> MAETKSMFREVLPKQGQLYVEDITTMVLCKPKLLPLKSLTLEKLEKMQQAAQDTIHQQEMTEKEQKITH;> MAATSSSDSDGGKGESEANSKWLDSLSDSMANIHTFSACLALADFHGDGEYKLAMGDLGPDGRQPRLKVLKGHTLVSQKPLPDLPAAAVTFLMASHEPRTPALAIASGPCVYVYKNLKPYFKFSLPSLPTNPLEQDLWNQAKEDQIDPLTLKEMLEGIREKAEVPLSVQSLRFLPLELSEMEAFVNQHKSKSIRRQTVITTMTTLKKNLADEDAVSCLVLGTENKELLVLDPEAFTILAKMSLPSVPAFLEASGQFDVEFRLAAACRNGSIYILRRDSKRPKYCIELGAQPVGLVGVHKVLVVGSNQDSLHGFTYKGKRLWTVQMPAAILAMNLLEQHSRGLQAVMAALANEEVRIYHDKVLLNVIRTPEAVTSLCFGRYGREDNTLIMTTLGGGLIIKILKRTAVFAEGGGEAGPPPSQAIKLNVPRKTRLYVDQTLREREAGTAMHRTFQADLYLLRLRAARAYVQALESSLSPVSLTAREPLKLHAVVQGLGPTFKLTLHLQNTSTARPILGLVVCFLYNEVLYALPRAFFKVPLLVPGLNYPLETFVKSLSDKGISDIIKVLVLREGQSTPLLSAHINMPMSEGLAAD;> MLQPVFTLKLRHKISPRMVAVGRYDGTHPCLAAATQAGKVFIHNPHSRSQHLGAPRVLQSPLESDVSLLNINQTVSCLTAGVLNPELGYDALLVGTQTNLLAYDVYNNSDLFYREVADGASAIVLGTLGDITSPLAIIGGNCALQGFNHEGNDLFWTVTGDNVHSLALCDFDGDGKKELLVGSEDFDIRVFKEDEIVAEMSETEIITSLCPMYGSRFGYALSNGTVGVYDKTARYWRIKSKNQAMSIHAFDLNSDGVCELITGWSNGKVDARSDRTGEVIFKDNFSSAIAGVVEGDYRMEGCQQLICCSVDGEIRGYLPGTAEMRGNLMDISVEQDLIRELSQKKQNLLLELRNYEENAKAELSSPLNEADGHRGVIPANTKHHTALSVSLGSEAQAAHAELCISTSNDTIIRAVLIFAEGVFAGESHVVHPSVHHLSSSVRIPITPPKDIPVDLHLKTFVGYRSSTQFHVFELTRQLPRFSMYALTSPDPASEPLSYVNFIIAERAQRVVMWLNQNFLLPEDTNIQNAPFQVCFTSLRNGGQLYIKIKLSGEITVNTDDIDLAGDIIQSMASFFAIEDLQVEADFPVYFEELRKVLVKVDEYHSVHQKLSADMADNSNLIRSLLVQAEDARLMRDMKTMKNRYKELYDLNKDLLNGYKIRCNNHTELLGSLKAVNQAIQRAGHLRVGKPKNQVITACRDAIRSNNINMLFRIMRVGTASS;> MAEEKLSARTQLPVSAESQKPVLKKAPEFPILEKQNWLIHLYYIQKDYEACKAVIKEQLQETHGLCEYAIYVQALIFRLEGNIQESLRLFQMCAFLSPQCADNLKQVARSLFLLGKHKAAIEVYNEAAKLNQKDWEICHNLGVCYIYLKQFDKAQDQLHNALHLNRHDLTYIMLGKIFLLKGDLDKAIEIYKKAVEFSPENTELLTTLGLLYLQLGIYQKAFEHLGNTLTYDPTNYKAILAAGSMMQTHGDFDVALTKYKVVACAVIESPPLWNNIGMCFFGKKKYVAAISCLKRANYLAPLDWKILYNLGLVHLTMQQYASAFHFLSAAINFQPKMGELYMLLAVALTNLEDSENAKRAYEEAVRLDKCNPLVNLNYAVLLYNQGEKRDALAQYQEMEKKVNLLKYSSSLEFDPEMVEVAQKLGAALQVGEALVWTKPVKDPKSKHQTASTSKAAGFQQPLGSNQALGQAMSSAATCRKLSSGAGGTSQLTKPPSLPLEPEPTVEAQPTEASAQTREK;> MSVLDALWEDRDVRFDVSSQQMKTRPGEVLIDCLDSVEDTKGNNGDRGRLLVTNLRIVWHSLALPRVNLSIGYNCILNITTRTANSKLRGQTEALYVLTKCNSTRFEFIFTNLVPGSPRLYTSLIAVHRAYETSKMYRDFKLRSALIQNKQLRLLPQENVYNKINGVWNLSSDQGNLGTFFITNVRIVWHANMNDSFNVSIPYLQIRSVKIRDSKFGLALVIESSQQSGGYVLGFKIDPVEKLQESVKEINSLHKVYSANPIFGVDYEMEEKPQPLEALTVKQIQDDVEIDSDDHTDAFVAYFADGNKQQDREPVFSEELGLAIEKLKDGFTLQGLWEVMN;> MDLNLNRADYLQVGVTSQKTMKLLPASKHRATQKVVVGDHDGIVMCFGMKKGEAVTVFKTLPGQKI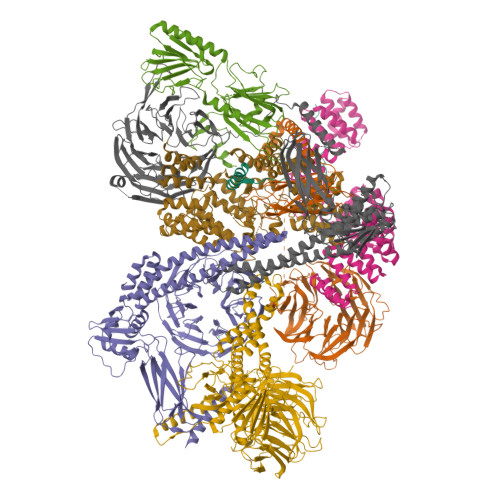ARLELGGALNTPQEKIFIAAGSEIRGFTKRGKQFLSFETNLTESIKAMHISGSDLFLSASYIYNHYCDCKDQHYYLSGDKINDVICLPVERLLREVPVLACQDRVLRVLQGSDVTYEIEVPGPPTVLALHNGNGGDSGEDLLFGTSDGKLGLIQITTSKPIHKWEIRNEKKRGGILCVDSFDIVGDGVKDLLVGRDDGMVEVYGFDNANEPVLRFDHTLSESVTSIQGGCVGKDGYDEIVVSTYSGWITGLTTEPVHKESGPGEELKFNQEMQNKISSLRSELEQLQYKVLQEREKYQQSSQSSKAKSAVPSFSVNDKFTLNKDDASYSLILEVQTAIDNVLIQSDVPIDLLDVDKNSAVVSFSSCDSESNDNFLLATYRCQANTTRLELKIRSIEGQYGTLQAYVTPRIQPKTCQVRQYHIKPLSLHQRTHFIDHDRPMNTLTLTGQFSFSELHSWVVFCMPEVPEKPPAGECVTFYFQNTFLDTQLESTYRKGEGVFKSDNISTISILKDVLSKEATKRKINLNISYEINEVSVKHTLKLIHPKLEYQLLLAKKVQLIDALKELQVHEGNTNFLIPEYRCILEEADHLQEEYKKQPAHLERLYGMITDLFIDKFKFKGTNVKTKVPLLLEILDSYDQNALIAFFDAA;> MEPLLLAWSYFRRRRFQLCADLCTQMLEKSPCDQAAWILKARALTEMVYVDEIDVDEEGIAEMILDENAIAQVPRPGTSLKLPGTNQTGGPSPAVRPVTQAGRPITGFLRPSTQSGRPGTIEQAIKTPRTAYTARPIASSSGRFVRLGTASMLTSPDGPFINLSRLNLAKYAQKPKLAKALFEYIFHHENDVKTALDLAALSTEHSQYKDWWWKVQIGKCYYRLGLYREAEKQFKSALKQQEMVDTFLYLAKVYISLDQPLTALNLFKQGLDKFPGEVTLLCGIARIYEEMNNISSATEYYKEVLKQDNTHVEAIACIGSNHFYTDQPEVALRFYRRLLQMGVYNCQLFNNLGLCCFYAQQYDMTLTSFERALSLAENEEEVADVWYNLGHVAVGTGDTNLAHQCFRLALVSNNQHAEAYNNLAVLEMRRGHVEQAKALLQTASSLAPHMYEPHFNFATISDKIGDLQRSYAAAKKSEAAFPDHVDTQHLIKQLEQHFAML;> MSLFKARDWWSTVLGDKEEFDQGCLCLADVDNTGNGQDKIIVGSFMGYLRIFNPHPVKTGDGAQAEDLLLEVHLRDPILQVEVGKFVSGTEMLHLAVLHSRKLCVYSVSGTLGNVEHGNQYQIKLMYEHNLQRTACNMTYGSFGGVKGRDLICIQSVDGMLMVFEQESYAFGRFLPGSLLPGPLAYSSRTDSFITVSSCHQVESYKYQVLAFATDADKRQETEQQKHGSGKRLVVDWTLNIGEQAIDICIVSFIQSASSVFVLGERNFFCLKDNGQIQFMKKLDYSPSCFLPYCSVSEGTINTLIGNHNNMLHIYQDVTLKWATQLPHVPVAVRVGCLHDLKGVIVTLSDDGHLQCSYLGTDPSLFQAPKVESRELNYDELDMELKELQKVIKNVNKSQDVWPLTEREDDLKVSAMVSPNFDSVSQATDVEVGADLVPSVTVKVTLKNRVALQKIKLSIYVQPPLVLTGDQFTFEFMAPEMTRTVGFSVYLKGSYSPPELEGNAVVSYSRPTERNPDGIPRVSQCKFRLPLKLVCLPGQPSKTASHKLTIDTNKSPVSLLSLFPGFAKQSEDDQVNVMGFRFLGGSQVTLLASKTSQRYRIQSEQFEDLWLITNELIIRLQEYFEKQGIKDFTCSFSGSVPLEEYFELIDHHFELRINGEKLEELLSERAVQFRAIQRRLLTRFKDKTPAPLQHLDTLLDGTYKQVIALADAVEENQDNLFQSFTRLKSATHLVILLIGLWQKLSADQIAILEAAFLPLQQDTQELGWEETVDAALSHLLKTCLSKSSKEQALNLNSQLGIPKDTSQLKKHITLFCDRLAKGGRLCLSTDAAAPQTMVMPGGCATIPESDLEGRSIDQDSSELFTNHKHLMVETPVPEVSPLQGVTE> SASEFNILNDGPPKETYVVDDAGVLSRVTKSDLKKLLSDLEYRKKLRLNFITVRKLTSKADAFEYADQVLEKWYPSIEEGNNKGIVVLITSQKEGAITGGPAFIEAVGENILDATVSENLPV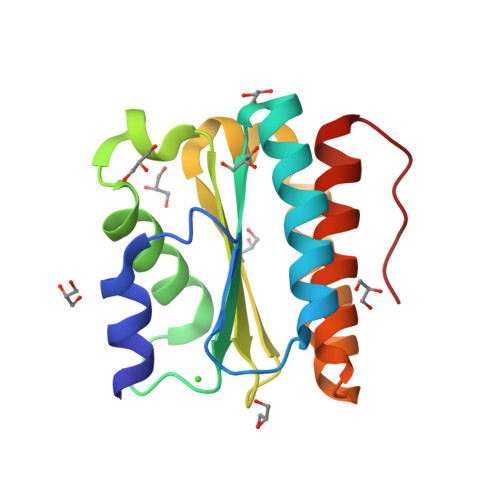LATDEKYNEAVYSSAKRLVAAIDGQPDPGGP> IGRLHKQ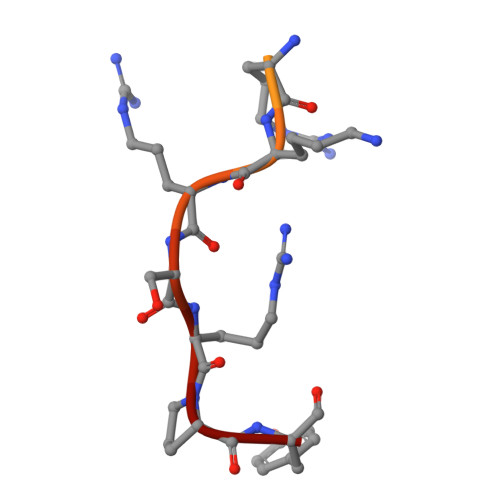RKPDRRKRSRPY> MADDFGFFSSSESGAPEAAEEDPAAAFLAQQESEIAGIENDEGFGAPAGSQGG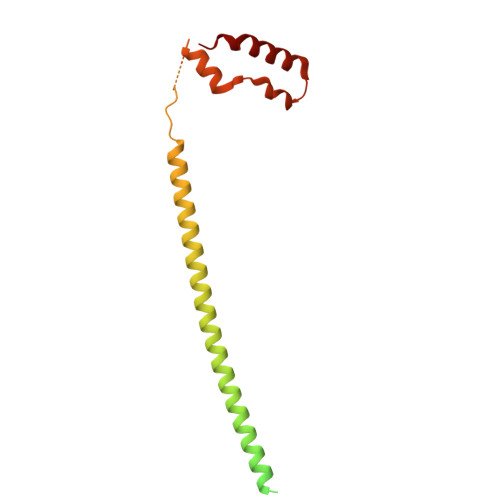LAQPGPASGASEDMGATVNGDVFQEANGPADGYAAIAQADRLTQEPESIRKWREEQRKRLQELDAASKVMEQEWREKAKKDLEEWNQRQSEQVEKNKINNRIADKAFYQQPDADIIGYVASEEAFVKESKEETPGTEWEKVAQLCDFNPKSSKQCKDVSRLRSVLMSLKQTPLSR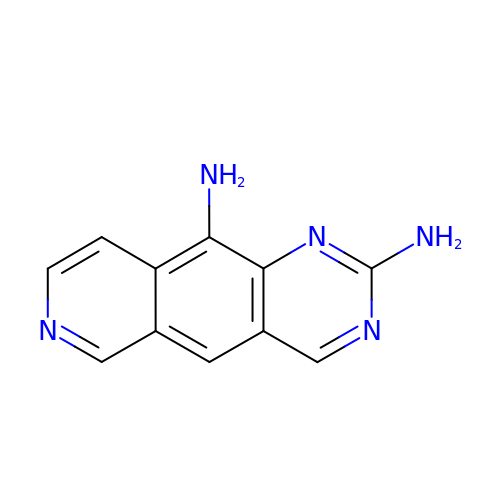pyrido[3,4-g]quinazoline-2,10-diamine | C11 H9 N5 | PQAQQDCVZZTPPJ-UHFFFAOYSA-N2'-DEOXYCYTIDINE-5'-TRIPHOSPHATE | C9 H16 N3 O13 P3 | 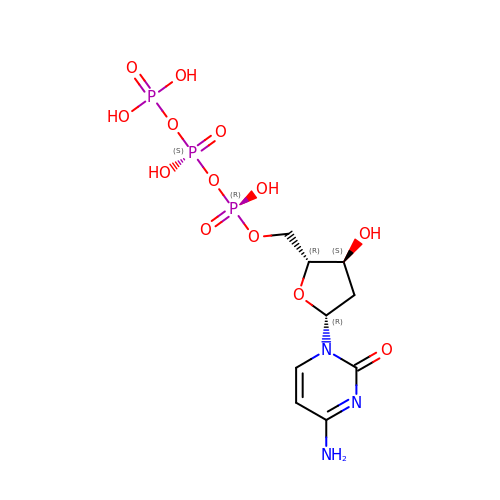RGWHQCVHVJXOKC-SHYZEUOFSA-N>[8x]MAGKLMHALQYNSYGGGAAGLEHVQVPVPTPKSNEVCLKLEATSLNPVDWKIQKGMIRPFLPRKFPCIPATDVAGEVVEVGSGVKNFKAGDKVVAVLSHLGGGGLAEFAVATEKLTVKRPQEVGAAEAAALPVAGLTALQALTNPAGLKLDGTGKKANILVTAASGGVGHYAVQLAKLANAHVTATCGARNIEFVKSLGADEVLDYKTPEGAALKSPSGKKYDAVVHCANGIPFSVFEPNLSENGKVIDITPGPNAMWTYAVKKITMSKKQLVPLLLIPKAENLEFMVNLVKEGKVKTVIDSKHPLSKAEDAWAKSIDGHATGKIIVEP

The chloroplast envelope Quinone Oxidoreductase Homolog (ceQORH; At4g13010; molecular weight 34,034 Da) from Arabidopsis thaliana is associated to the inner membrane of the chloroplast envelope where it represents 1–2% of the crude envelope proteins. Despite its original annotation as a “QOR,” ceQORH is inactive on quinones but preferentially reduces γ-ketols in the presence of NADPH. γ-ketols are long-chain reactive electrophile oxylipins and are potentially toxic. The ceQORH monomer is formed of two domains with (i) the catalytic domain including residues from Gly3 to Pro132 and from Leu277 to Pro329 and (ii) the cofactor binding domain (Val133 to Leu276) showing the classical motif of Rossmann fold. In the ceQORH structure, the internal chloroplast targeting sequence is folded as a two anti-parallel β-strands (Thr71 to Gly81 and Asp91 to Leu97) connected by a long loop (Ser82 to Gly90).

In the crystals of the binary and ternary complexes ceQORH-13-KOTE and ceQORH-NADP+-13-KOTE, the asymmetric unit contains 12 and 8 ceQORH molecules, respectively. NADP+ is bound at the interface of the two domains and the nicotinamide ring is in the vicinity of the catalytic site. Comparison of apo-ceQORH and ceQORH-NADP+-13-KOTE monomers shows that NADP+ binding introduces local changes in the vicinity of the cofactor. The orientation of the Arg190 side chain is modified, stabilizing the 2′-phosphate of the NADP+ adenosine moiety. The loop containing Thr251 in the Rossmann fold shifts and stabilizes the ribose group of the NADP+ nicotinamide moiety by interacting with the Thr251 hydroxyl group. In the ceQORH-NADP+-13-KOTE structure, the aliphatic chain of 13-KOTE is observed in electron density up to the C11 atom of the α,β-unsaturated carbon-carbon bond (C11 = C12). The distance average between the C11 atom and the C4 atom of the NADP+ nicotinamide ring bearing the hydride is 6.84 Å. The flexibility of 13-KOTE and the large distance between the α,β-unsaturated carbon-carbon bond (C11 = C12) and the C4 atom of NADP+ nicotinamide ring are not compatible with a hydride transfer. The new position of the α-helix Pro254-Met267 observed in ceQORH-NADP+-13-KOTE could prevent the dimer formation when ceQORH binds NADPH and may explain why ceQORH-NADPH behaves as a monomer in solution (Mas y mas et al., 2015).> VREILSIHVGQCGNQIADSFWRLALREHGLTEAGTLKEGSNAAANSNMEVFFHKVRDGKYVPRAVLVDLEPGVIARIEGGDMSQLFDESSIVRKIPGAANNWARGYNVEGEKVIDQIMNVIDSAVEKTKGLQGFLMTHSIGGGSGSGLGSLILERLRQAYPKKRIFTFSVVPSPLISDSAVEPYNAILTLQR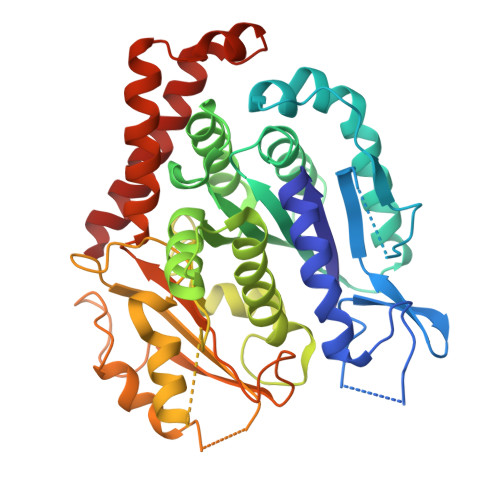ILDNADGAVLLDNEALFRIAKAKLNRSPNYMDLNNIIALIVSSVTASLRFPGKLNTDLSEFVTNLVPFPGNHFLTASFAPMRGAGQEGQVRTNFPDLARETFAQDNFTAAIDWQQGVYLAASALFRGDVKAKDVDENMATIRKSLNYASYMPASGGLKLGYAETAPEGFASSGLALVNHTGIAAVFERLIAQFDIMFDNHAYTHWYENAGVSRDMMAKARNQIATLAQSYRDAS> MELHQIRGCHKNDIELKKYNIGVAISLGNKWFSIDNIEKLVKWSLLHTKEYVIIYIADSIHGINLSVRNKLSDSHAEEVAIRYGRNLFIKIKERVSLSFSQDEQAKIIYATWSDIADSKYKEKVKYLYNLYDKNINFKNYIENFVKEWVSKEKRTFNNNEINKFGRYILEQLPELMVQVKARGVLFEAYVYPYKTRITEFVGLLQKGEIFPEIKTNILDNHPKIFLEVRE

Cyclodipeptide synthases (CDPSs) use aminoacylated tRNA (aa-tRNA) substrates to form peptide bonds between two amino acids yielding a cyclic dipeptide product (CDP). ParaCDPS from Parabacteroides sp. 20_3 (GenBank: EFK64745.1) produces cyclo(His-Phe)8 whilst ParcuCDPS from Parcubacteria bacterium RAAC4_OD1_1 (GenBank: ETB63777.1) can synthesise both cyclo(His-Glu) and cyclo(His-Pro)9. ParcuCDPS belongs to the XYP sub-group of the CDPS family, characterised by the presence of 3 residues: X40 where X is a non-conserved residue, Y202, and P203 (numbering respective to AlbC). ParcuCDPS displays a Rossman-fold common throughout the CDPS family.

The active site includes the four conserved residues previously identified: S26, Y167, E171 and Y191. Previous research by us and others has shown that mutations in active site residues seriously reduce product formation in CDPS enzymes. The active site mutants – S26A; S26C; D58A; D58N; Y167A; Y167F; E171A; and E171Q—were also generated to confirm the loss of activity upon removing catalytic residues. Further investigation into the changes imposed by these mutants was performed by solving the crystal structures of a select few mutants containing changes to the active site or the pocket residues. The mutant structures were able to be solved using WT as a model and retained an equivalent fold to ParcuCDPS (Supplementary Notes 4 and 7 relating to Supplementary Figs. 13 and 14). Therefore, the disruption of activity is caused exclusively by the change in these few residues which appear important for the enzyme to produce a CDP.> HHHHHHMNASPTPTATTTTEPATAVVRCRTRLARRVVAAVGPDGLLPAPCESRVLESALALALLTEERAEADATARLTAYLRTTLRTAPPDPFQCAVARAVLGGAGERGERVGDEGDMDAGTALDAGLDGFDHFTAGRKRLMFRTVLAALGATGFPAVPWEAYDTRPQQSWLHMEMKALKVLAAHGTGHPDVVRDEDWRALLPALEPGPAWECNNLAQLLALLALRHSPRHRPALGDVLKHVAGRLRPDGGMPAIDGMTVFTTAAAGLALSLLPAPPACVTPMADALALRRNPDGGYGFHSGVAQSDVEDTCYVLEFLRRAAPDRHRTAVAEAEGYLLALRNPDGGFPTFARGTSSEIAMTAAAASALAHDPDRREEVDEAVRYVVRHQR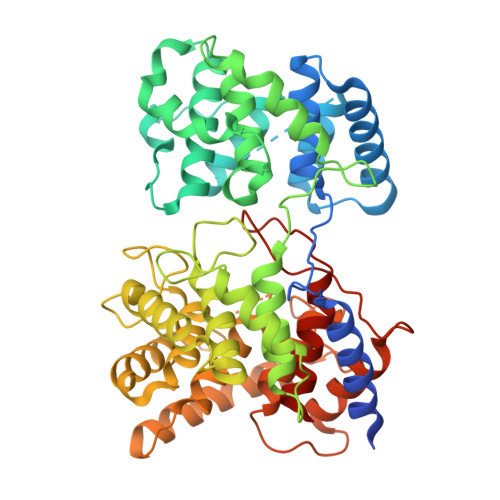PDGTFERSWSRNATNAVFRAVLALTGVAAHGEERRSRARAAERALAHLAATQNGDGGWGHAEAEPSDPISTAYAVIALARGPRARPGGPLDRALAYLVERQHPDGGYRSRPDQAGPRPLLYDVPALADVFVLLALAHATATPDPEGCSR>SKVYTAKGIRDRRVRLSVSTAIQFYDLQDRLGYDQPSKAIEWLIKA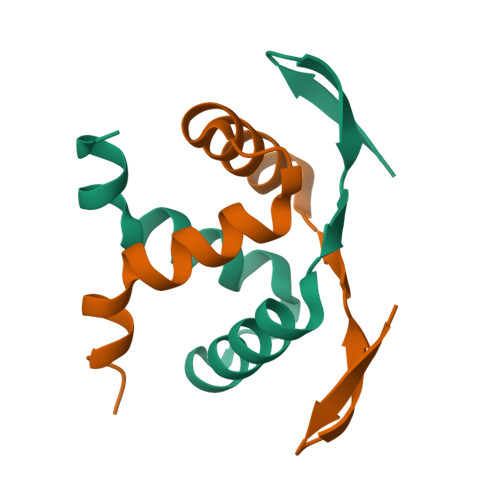AAAAIDKLP[2x]>XMFIVNTNVPRASVPDGFLSELTQQLAQATGKPPQYIAVHVVPDQLMAFGGSSEPCALCSLHSIGKIGGA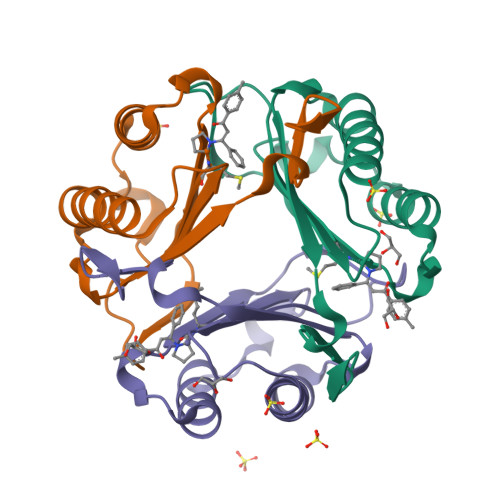QNRSYSKLLCGLLAERLRISPDRVYINYYDMNAANVGWNNSTFA[6x]2-ACETYLAMINO-7-(1,2-DIHYDROXY-ETHYL)-3-HYDROXY-6,8-DIOXA-BICYCLO[3.2.1]OCTANE-5-CARBOXYLIC ACID | C11 H17 N O8 | 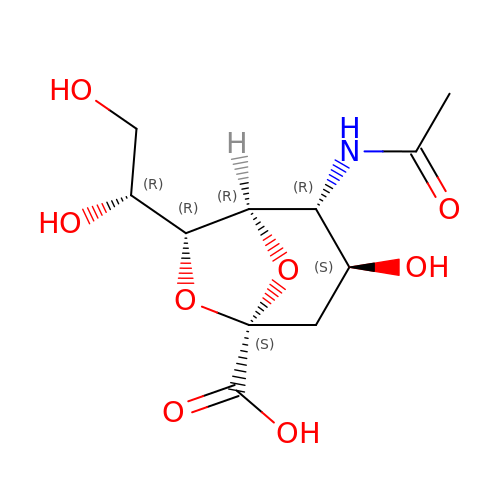NCMJSVDTRDLWJE-YRMXFSIDSA-N> VVGGTRAAQGEFPFMVRLINEENEGFCGGALYAQDIVLTAAHCVSGSGNNTSITATGGVVDLQSSSAVKVRSTKVLQAPGFTKETYGKDWALIKLAQPINQPTLKIAT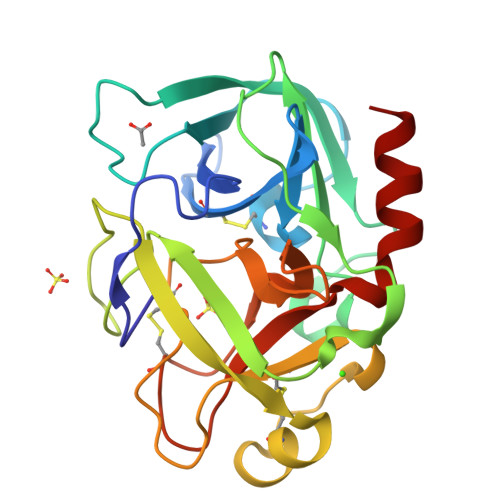TTAYNQGTFTVAGWGANREGGSQQRYLLKANVPFVSDAACRSSSSFILVANEMICAGYPDTGGVDTCQGDSGGPMFRKDNADEWIQVGIVSWGYGCARPGYPGVYTEVSTFASAIASAARTL>MPKSEIRKLLQEIKKQVDNPGNSSTTEIKKMASEAGIDEQTAEEIYHLLTEFYQAVEEHGGIEKYMHSNISWLKIELELLSACYQIAILEDMKVLDISEMLSLNDLRIFPKTPSQLQNTYYKLKKELIQVEDIPKNKPGRKRKTQKNTKKEKTNIFGKVVPALE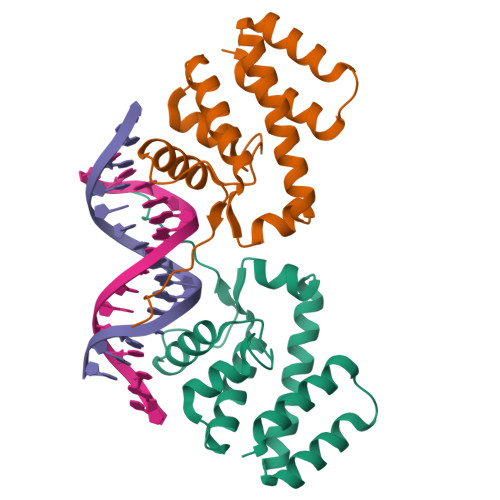HHHHHH[2x]> NPVERYVDEVLNEVLVVPNINQSHPTTSNAAPVLDAAETGHTNKIQPEDTIETRYVQSSQTLDEMSVESFLGRSGCIHESVLDIVDNYNDQSFTKWNINLQEMAQIRRKFEMFTYARFDSEITMVPSVAAKDGHIGHIVMQYMYVPPGAPIPTTRDDYAWQSGTNASVFWQHGQPFPRFSLPFLSIASAYYMFYDGYDGDTYKSRYGTVVTNDMGTLCSRIVTSEQLHKVKVVTRIYHKAKHTKAWCPRPPRAVQYSHTHTTNYKLSSEVHNDVAIRPRTNLTTV;> SPSVEACGYSDRIIQITRGDSTITSQDVANAVVGYGVWPHYLTPQDATAIDKPTQPDTSSNRFYTLDSKMWNSTSKGWWWKLPDALKDMGIFGENM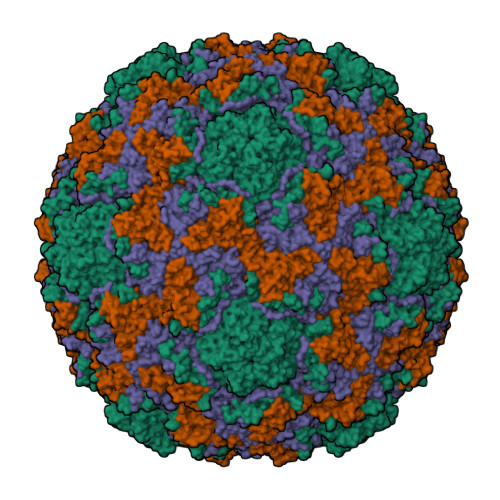FYHFLGRSGYTVHVQCNASKFHQGTLLVVMIPEHQLATVNKGNVNAGYKYTHPGEAGREVGTQVENEKQPSDDNWLNFDGTLLGNLLIFPHQFINLRSNNSATLIVPYVNAVPMDSMVRHNNWSLVIIPVCQLQSNNISNIVPITVSISPMCAEFSGARAKTVVQ;> GLPVYVTPGSGQFMTTDDMQSPCALPWYHPTKEIFIPGEVKNLIEMCQVDTLIPINSTQSNIGNVSMYTVTLSPQTKLAEEIFAIKVDIASHPLATTLIGEIASYFTHWTGSLRFSFMFCGTANTTLKVLLAYTPPGIGKPRSRKEAMLGTHVVWDVGLQSTVSLVVPWISASQYRFTTPDTYSSAGYITCWYQTNFVVPPNTPNTAEMLCFVSGCKDFCLRMARDTDLHKQTGPITQ;> GAQVSRQNVGTHSTQNMVSNGSSLNYFNINYFKDAASSGASRLDFSQDPSKFTDPVKDVLEKGIPTLQ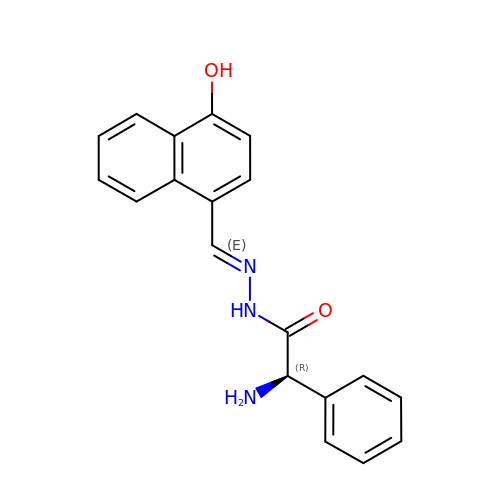(2R)-2-amino-N'-[(E)-(4-hydroxynaphthalen-1-yl)methylidene]-2-phenylethanehydrazide | C19 H17 N3 O2 | WWYPXPWOVWOANL-AGKWGAAGSA-N>MVDYSDCFEGISGGAIFYNTKNKEYNIYNKELIETRRSPCSTFKIVSTLIGLEKGVINSKESVMGYDGTEYPNKNWNKNLSLEEAFKESCVWYYKK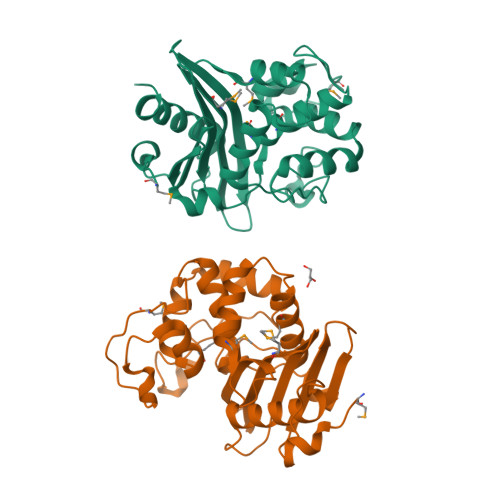LIDKVDAKSVQNILDDLKYGNCDISEWEGDLKNGKGHLNGFWLESSLQISPKEQVQTMAKIFEGDTNFKKEHINILRDIMKIDVNDKNINVYGKTGTGFDEKNKRVDAWFVGMLEREGDTYYFAIKSDDSNKEITGPKVKEIAINIIKKYYSVREGAAL[4x]> MDRKVAREFRHKVDFL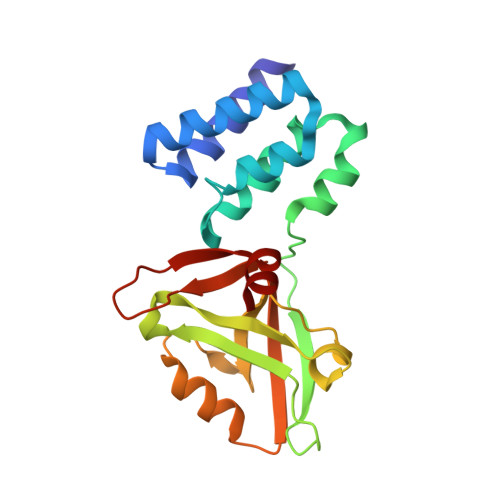IENDAEKDYLYDVLRMYHQTMDVAVLVGDLKLVINEPSRLPLFDAIRPLIPLKHQVEYDQLTPRRSRKLKEVRLDRLHPEGLGLSVRGGLEFGCGLFISHLIKGGQADSVGLQVGDEIVRINGYSISSCTHEEVINLIRTEKTVSIKVRHIGLIPVKSSPDEPLTWQYVDQFVSES>[4x]GSHMEQFDFDVVIVGGGPAGCTCALYTARSELKTVILDKNPAAGALAITHKIANYPGVPGEMSGDHLLEVMRDQAVEFGTVYRRAQVYGLDLSEPVKKVYTPEGIFTGRALVLATGAMGRIASIPGEAEYLGRGVSYCATCDGAFYRNREVVVVGLNPEAVEEA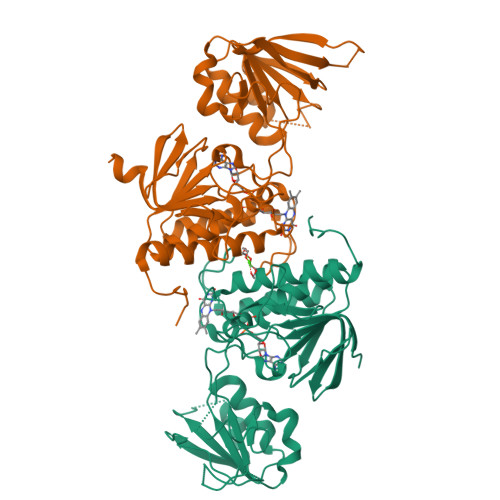QVLTKFASTVHWITPKDPHTLDGHADELLAHPSVKLWEKTRLIRIKGEEAGVTAVEVRHPGESDSQELLAEGVFVYLQGSKPITDFVAGQVEMKPDGGVWVDEMMQTSVPGVWGIGDIRNTPFKQAVVAAGDGCIAAMAIDRFLNSRKAIKPDWAH>GSQDSTSDLIPAPPLSKVPLQQNFQDNQFQGKWYVVGLAGNAILREDKDPQKMYATIYELKEDKSYNVTSVLFRKKKCDYWIRTFVPGSQPGEFTLGNIKSYPGLTSYLVRVVSTNYNQHAMVFFKKVSQNREYFKITLYGRTKELTSELKENFIRFSKSLGLPENHIVFPVPIDQC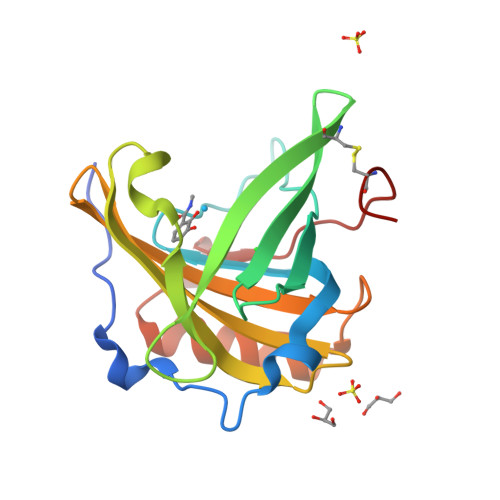IDG[3x]>[2x]GAMETITVPTPIKQIFSDDAFAETIKDNLKKKSVTDAVTQNELNSIDQIIANNSDIKSVQGIQYLPNVTKLFLNGNKLTDIKPLANLKNLGWLFLDENKVKDLSSLKDLKKLKSLSLEHNGISDINGLVHLPQLESLYLGNNKITDITVLSRLTKLDTLSLEDNQISDIVPLAGLTKLQNLYLSKNHISDLRALAGLKNLDVLELFSQECLNKPINHQSNLVVPNTVKNTDGSLVTPEIISDDGDYEKPNVKWHLPEFTNEVSFIFYQPVTIGKAKARFHGRVTQPLKE;>ETRECKEALAKSEMNVNMKCQLPNFTAETPIQNVILHEHHIFLGATNYIYVLNEEDLQKVAEYKTGPVLEHPDCFPCQDCSSKANLSGGVWKDNINMALVVDTYYDDQLISCGSVNRGTCQRHVFPHNHTADIQSEVHCIFSPQIEEPSQCPDCVVSALGAKVLSSVKDRFINFFVGNTINSSYFPDHPLHSISVRRLKETKDGFMFLTDQSYIDVLPEFRDSYPIKYVHAFESNNFIYFLTVQRETLDAQTFHTRIIRFCSINSGLHSYMEMPLECILTEKRKKRSTKKEVFNILQAAYVSKPGAQLARQIGASLNDDILFAVFAQSKPDSAEPMDRSAMCAFPIKYVNDFFNKIVNKNNVRCLQHFYGPNHEHCFNRTLLRNSSGCEARRDEYRTEFTTALQRVDLFMGQFSEVLLTSISTFIKGDLTIANLGTSEGRFMQVVVSRSGPSTPHVNFLLDSHPVSPEVIVEHTLNQNGYTLVITGKKITKIPLNGLGCRHFQSCSQCLSAPPFVQCGWCHDKCVRSEECLSGTWTQQICLPAIYKVFPNSAPLEGGTRLTICGWDFGFRRNNKFDLKKT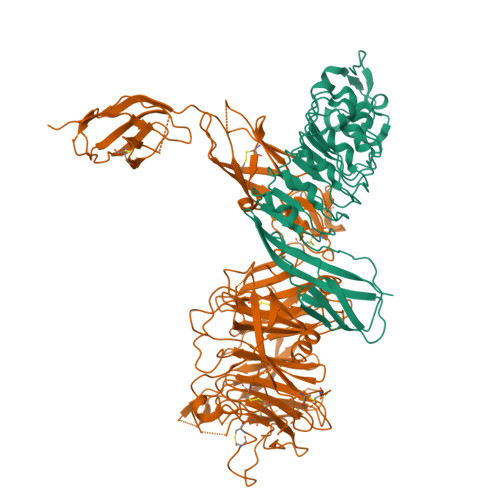RVLLGNESCTLTLSESTMNTLKCTVGPAMNKHFNMSIIISNGHGTTQYSTFSYVDPVITSISPKYGPMAGGTLLTLTGNYLNSGNSRHISIGGKTCTLKSVSNSILECYTPAQTISTEFAVKLKIDLANRETSIFSYREDLHHHHHH[2x]> MVTSNVVLVSGEGERFTVDKKIAERSLLLKNYLND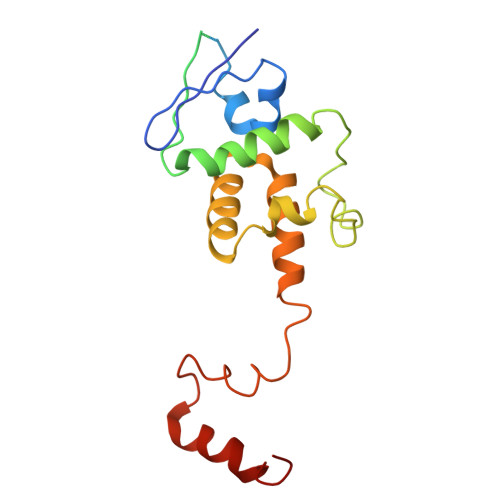MHDSNLQNNSDSESDSDSETNHKSKDNNNGDDDDEDDDEIVMPVPNVRSSVLQKVIEWAEHHRDSNFPDEDDDDSRKSAPVDSWDREFLKVDQEMLYEIILAANYLNIKPLLDAGCKVVAEMIRGRSPEEIRRTFNIVNDFTPEEEAAIRRENEWAEDR> MRLLYLHADRFEYKTVKPALKNPPDPPGEASFGEALVVFTTVEDGDGPQ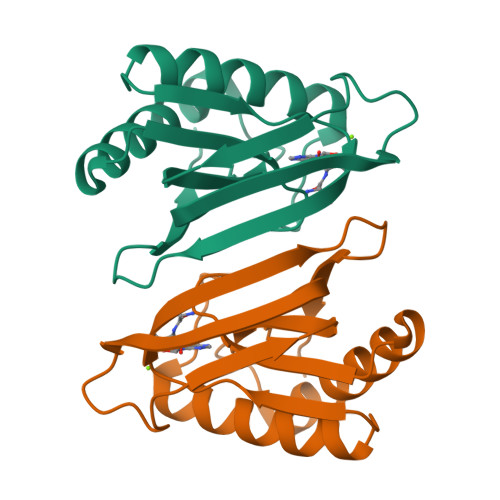TVMYAASDIASHSSRLKVTTVILYPYAHLSSRLAKPMAAHKRLIELEGALRTKFPGHVHRAPFGWYMSFSIACKGHPLAELSRSFTE>[4x]GMDYQEYQQFLARINTARDACVAKDIDVDLLMARHDYFGRELCKSLNIEYRNDVPFIDIILDIRPEVDPLTIDAPHITPDNYLYINNVLYIIDYKVSVSNESSVITYDKYYEL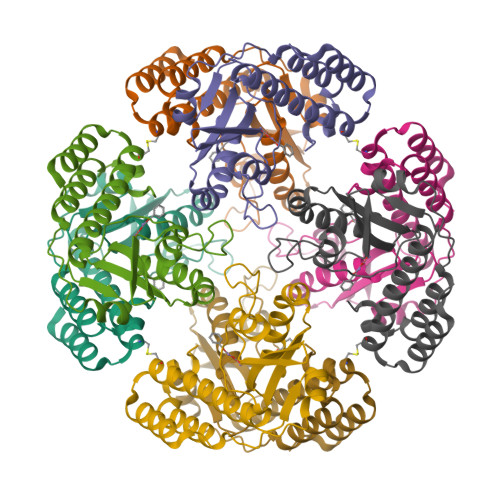TRDISDRLSIPIEIVIIRIDPVSRDLHINSDRFKELYPTIVVDINFNQFFDLKQLLYEKFGDDEEFLLKVA NAPHTHALENE-1,2-DIOL | C10 H8 O2 | 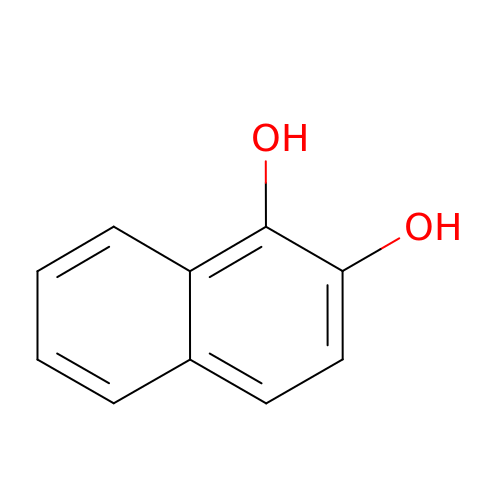NXPPAOGUKPJVDI-UHFFFAOYSA-N> QGTREQLNLCLERLSSGKDKNKSVLQNKYVRC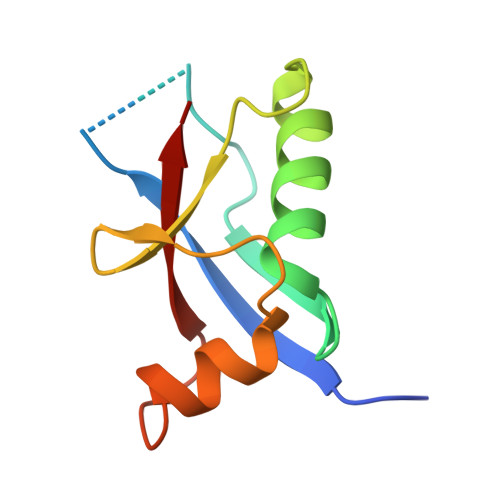SVRAEVRHLRRVLCHRLMLNPQHVQLLFDNEVLPDHMTMKQIWLSRWFGKPSPLLLQYSVK cyclobutyl-[4-(2-methoxyphenyl)piperidin-1-yl]methanone 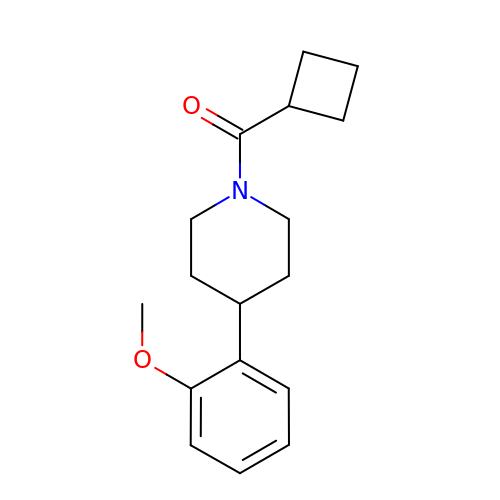| C17 H23 N O2 | QTCJMGOUQOSHRR-UHFFFAOYSA-N> SNAMQR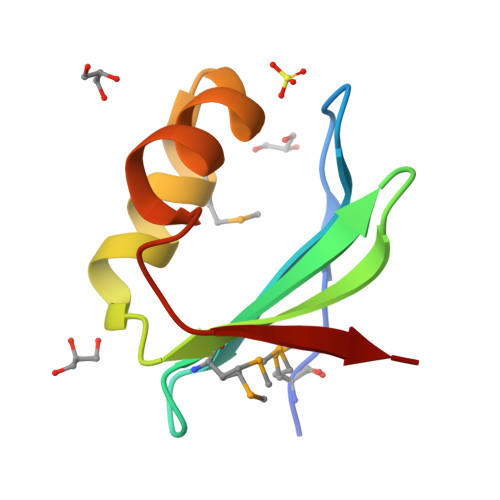QPVSSSRILSIGYDPDNRMLEIQFREQGTYQYLGVPERAHQNFMSAVSKGRFFDGVIKGKFLCRKIG> MTKRVRLSDSFNPVYPYEDESTSQHPFINPGFISPNGFTQSPNGVLTLKCLTPLTTTGGSLQLKVGGGLTVDDTNGFLKENISATTPLVKTGHSIGLPLGAGLGTNENKLCIKLGQGLTFNSNNICIDDNINTLWTGVNPTEANCQIMNSSESNDCKLILTLVKTGALVTAFVYVIGVSNNFNMLTTHRNINFTAELFFDSTGNLLTRLSSLKTPLNHKSGQNMATGAITNAKGFMPSTTAYPFND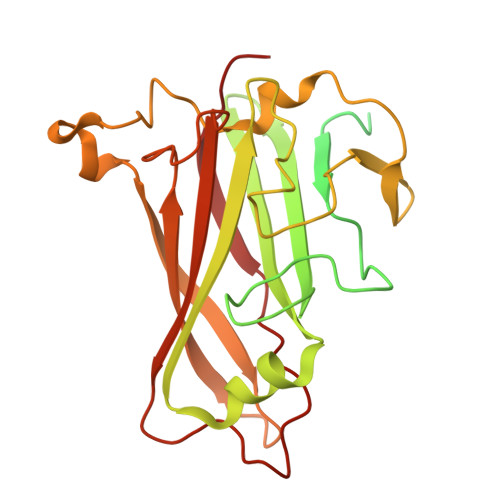NSREKENYIYGTCYYTASDRTAFPIDISVMLNRRAINDETSYCIRITWSWNTGDAPEVQTSATTLVTSPFTFYYIREDD> ADLANGAKVFSGNCAACHMGGGNVV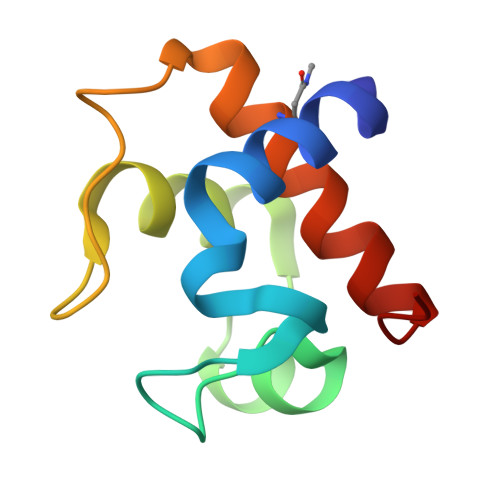MANKTLKKEALEQFGMYSEEAIIYQVQHGKNAMPAFAGRLTDEQIQNVAAYVLDQAAKGWAG>[2x]MMSVQKANTVSRQKATGAHFTPDKLAEVIAKRILDYFKGEKNRVIRVLDPACGDGELLLAINKVAQSMNIQLELIGVDFDIDAINIANERLSRSGHKNFRLINKDFLEMVSEGDNYDLFNIEELEPVDIIIANPPYVRTQILGAEKAQKLREKFNLKGRVDLYQAFLVAMTQQLKSNGIIGVITSNRYLTTKGGESTRKFLVSNFNILEIMDLGDSKFFEAAVLPAIFFGEKKNKEYQKENSNVPKFFKIYEQSDIEASSSVNSEFNSLIELLEVNKSGLYSVEDKTYSISLGKIISPENYKEPWILATEDEYEWFMKVNQNAYGFIEDFAHVKVGIKTTADSV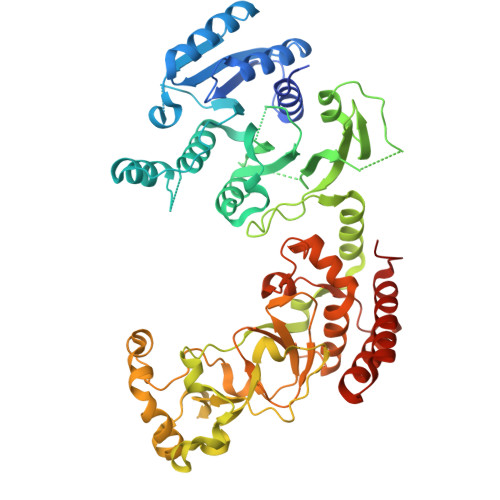FIRSDWGELPEEQIPEDKLLRPIISADQANKWSVSLVGNNKKVLYTHEIRDGQIKAINLEEFPRAKNYLESHKERLASRKYVLKANRNWYEIWVPHDPSLWDKPKIIFPDTSPEPKFFYEDKGSVVDGNCYWIIPKKENSNDILFLIMGICNSKFMSKYHDIAFQNKLYAGRRRYLTQYVNKYPIPDPESIYSKEIISLVRELVNNKKETQDINEIENRIEKLILRAFDIESLKYHHHHHH>[2x]MVLYFIGLGLYDERDITVKGLEIAKKCDYVFAEFYTSLMAGTTLGRIQKLIGKEIRVLSREDVELNFENIVLPLAKENDVAFLTPGDPLVATTH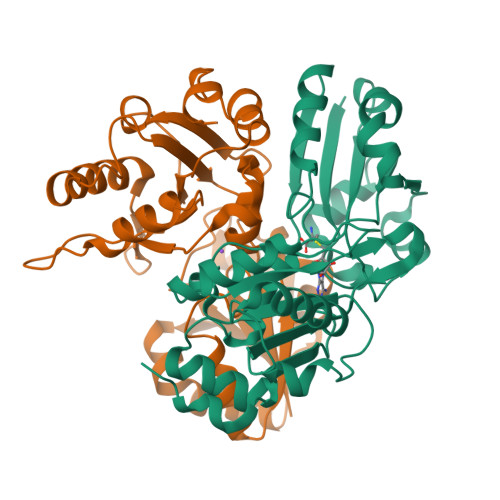AELRIRAKRAGVESYVIHAPSIYSAVGITGLHIYKFGKSATVAYPEGNWFPTSYYDVIKENAERGLHTLLFLDIKAEKRMYMTANEAMELMLKVEDMKKGGVFTDDTLVVVLARAGSLNPTIRAGYVKDLIREDFGDPPHILIVPGKLHIVEAEYLVEIAGAPREILRVNV>[2x]TDTFQMFWLDYCEVNNTLILFGKVKLKDDNCVSAMVQINGLCRELFFLPREGKTPTDIHEEIIPLLMDKYGLDNIRAKPQKMKYSFELPDIPSESDYLKVLLPYQTPKSSRDTIPSDLSSDTFYHVFGGNSNIFESFVIQ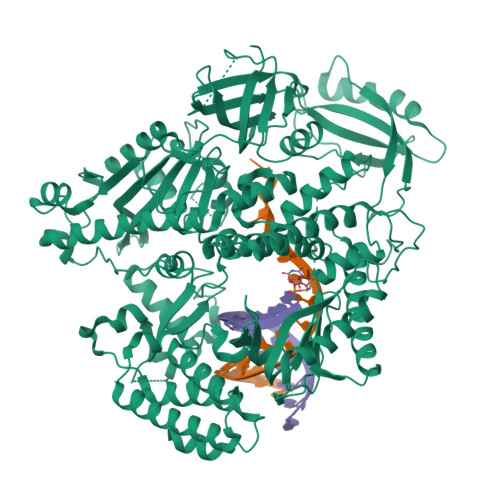NRIMGPCWLDIKGADFNSIAAASHCAVEVSVDKPQNITPTTTKTMPNLRCLSLSIQTLMNPKENKQEIVSITLSAYRNISLDSPIPENIKPDDLCTLVRPPQSTSFPLGLAALAKQKLPGRVRLFNNEKAMLSCFCAMLKVEDPDVIIGHRLQNVYLDVLAHRMHDLNIPTFSSIGRRLRRTWPEKFGRGNSNMNHFFISDICSGRLICDIANEMGQSLTPKCQSWDLSEMYQVTCEKEHKPLDIDYQNPQYQNDVNSMTMALQENITNCMISAEVSYRIQLLTLTKQLTNLAGNAWAQTLGGTRAGRNEYILLHEFSRNGFIVPDKEGNRSRAQKQRQNEENADAPVNSKKAKYQGGLVFEPEKGLHKNYVLVMDFNSLYPSIIQEFNICFTTVDRNKEDIDELPSVPPSEVDQGVLPRLLANLVDRRREVKKVMKTETDPHKRVQCDIRQQALKLTANSMYGCLGYVNSRFYAKPLAMLVTNKGREILMNTRQLAESMNLLVVYGDTNSVMIDTGCDNYADAIKIGLGFKRLVNERYRLLEIDIDNVFKKLLLHAKKKYAALTVNLDKNGNGTTVLEVKGLDMKRREFCPLSRDVSIHVLNTILSDKDPEEALQEVYDYLEDIRIKVETNNIRIDKYKINMKLSKDPKAYPGGKNMPAVQVALRMRKAGRVVKAGSVITFVITKQDEIDNAADTPALSVAERAHALNEVMIKSNNLIPDPQYYLEKQIFAPVERLLERIDSFNVVRLSEALGLDSKKYFRREGGNNNG>MKKVIIAGNGPSLKEIDYSRLPNDFDVFRCNQFYFEDKYYLGKKCKAVFYNPSLFFEQYYTLKHLIQNQEYETELIMCSNYNQAHLENENFVKTFY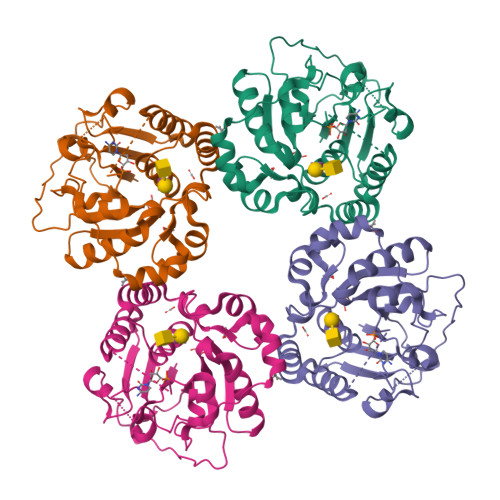DYFPDAHLGYDFFKQLKDFNAYFKFHEIYFNQRITSGVYMCAVAIALGYKEIYLSGIDFYQNGSSYAFDTKQKNLLKLAPNFKNDNSHYIGHSKNTDIKALEFLEKTYKIKLYCLCPNSLLANFIGLAPNLNSNFIIQEKNNYTKDILIPSSEAYGKFSKNI[2x]(2Z)-3,3,3-trifluoro-2-(hydroxyimino)propanoic acid | C3 H2 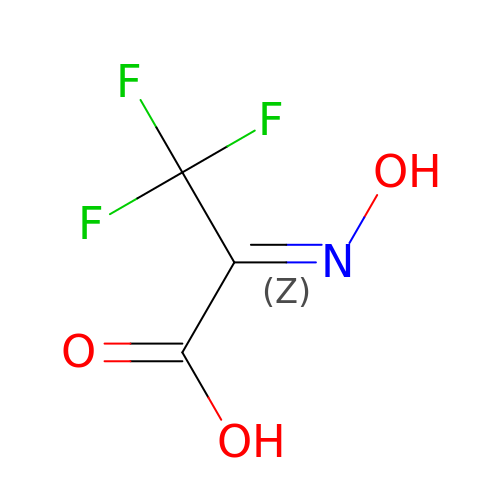F3 N O3 | ABQHLJFPKHMBRJ-XFSBKJJWSA-N> KTLVYCSEGSPEGFNPQLFISGTTYDASSVPLYNRLVEFKIGTTEVIPGLAEKWEVSEDGKTYTFHLRKGVKWHDNKEFKPTRELNADDVVFSFDRQKNAQNPYHKVSGGSYEYFEGMGLPELISEVKKVDDNTVQFVLTRPEAPFLADLAMDFASILSKEYADAMMKAGTPEKLDLNPIGTGPFQLQQYQKDSRIRYKAFDGYWGTKPQIDTLVFSITPDASVRYAKLQKNECQVMPYPNPADIARMKQDKSINLMEMPGLNVGYLSYNVQKKPLDDVKVRQALTYAVNKDAIIKAVYQGAGVSAKNLIPPTMWGYNDDVQDYTYDPEKAKALLKEAGLEKGFSIDLWAMPVQRPYNPNARRMAEMIQADWAKVGVQAKIVTYEWGEYLK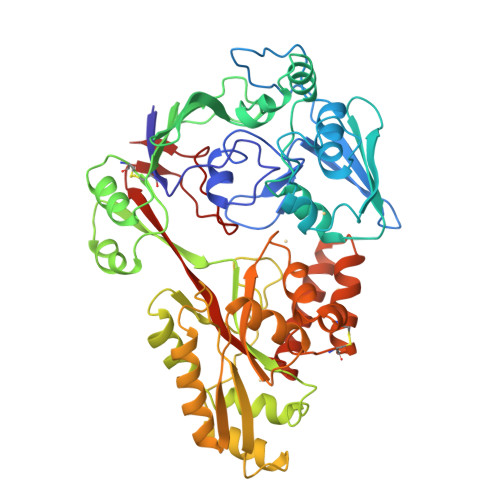RAKDGEHQTVMMGWTGDNGDPDNFFATEFSCAASEQGSNYSKWCYKPFEDLIQPARATDDHNKRVELYKQAQVVMHDQAPALIIAHSTVFEPVRKEVKGYVVDPLGKHHFENVSIE> MDIQLFSKTPSVTVFDNRGLSVRDIAYRRHPDTPKVTEECITYHQFDFRGFLAQSLDPRLNHKEVTNFSYLTDLNGNIIYTQSVDAGNTLVLNDTEGRSVIAMTNISRGENGKDDLSLAVTRTFQYENAPLPGRPLSVTEQVNGENARITEHFVYAGNTPQEKNLNLAGQCVSYYDAAGLIQTDSVSLTGKPLSVSRKLLKNLDDTNILADWQGNDTSAWNSLLATEIYTTVTRTDAAGAVLTTIDAVGNQQRVAFDIAGQLSASWLTLKGGQEQVIIKVLTYSAAGQKLREEGGNGVVTTYTYEAETQRLIGIKTERPNGHAAGAKVLQDLRYEYDPVGNVLSITNDAEETRFWRNQKVVPENAYRYDSLYQLVSASGREVAGAGQQGSDLPSPLVPLPSDSSVYTNYTRTYTYDSAGNLMRIRHSAPATNNNYTLNITVSERSNRGVMSSLTENPADVDALFTASGSQKCLQQGQSLIWTPRGELRTVLLVARGETADDSESYRYDGSSQRILKI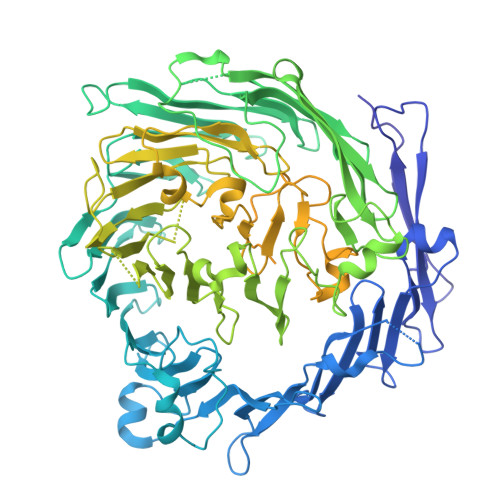SSQQTNHSARVQRALYLPGLEWRTMTGGVAEAENLQVICIGEAGRAQVRVLHWESGKPDGIINDQIRWSYDNLTCSSGLEVDGDGLVISMEEYYPYGGTAVWAARSHIETAYKTVRYSGKERDATGLYYYGFRYYQPWAGRWLSADPAGTVDGLNLYRMVRNNPLRLTDPDGMAPLDWLDLDTTNASRDIVKAIYQLNQIDGPHRGVRDTYQRMTESTGMILQETLNNEAVLKGIKQKDKEKKSRGMKFTNSKLKTYAAHAGVLNTLQPDPVYKDGFLNLPGSLGNKNTFPGVELIEDKVKPSLSQYHPDKLGKSQRWKPESSLGYYRVADTEAFITGIRSQYKSSGTDLHAVVEGRIRDHLLANNNVLPKMAGIAGLHAEVQALNYIISNPDIEGGNAERLNGSYIFTQRLVGDVNQDFPACYNCSGIISGLENVMTGRVNNDVRLKRRKSF>YNLDVRGARSFSPPRAGRHFGYRVLQVGNGVIVGAPGEGNSTGSLYQCQSGTGHCLPVTLRGSNYTSKYLGMTLATDPTDGSILACDPGLSRTCDQNTYLSGLCYLFRQNLQGPMLQGRPGFQECIKGNVDLVFLFDGSMSLQPDEFQKILDFMKDVMKKLSNTSYQFAAVQFSTSYKTEFDFSDYVKWKDPDALLKHVKHMLLLTNTFGAINYVATEVFREELGA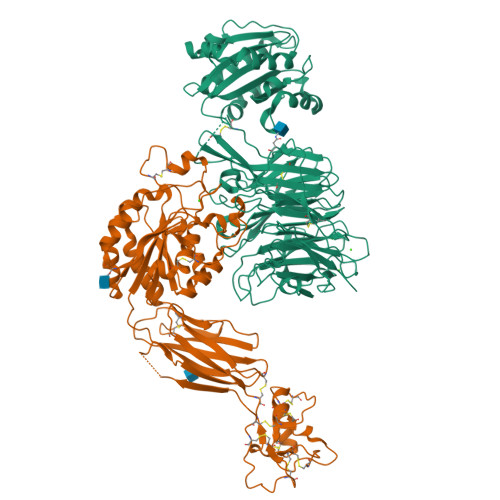RPDATKVLIIITDGEATDSGNIDAAKDIIRYIIGIGKHFQTKESQETLHKFASKPASEFVKILDTFEKLKDLFTELQKKIYVIEGTSKQDLTSFNMELSSSGISADLSRGHAVVGAVGAKDWAGGFLDLKADLQDDTFIGNEPLTPEVRAGYLGYTVTWLPSRQKTSLLASGAPRYQHMGRVLLFQEPQGGGHWSQVQTIHGTQIGSYFGGELCGVDVDQDGETELLLIGAPLFYGEQRGGRVFIYQRRQLGFEEVSELQGDPGYPLGRFGEAITALTDINGDGLVDVAVGAPLEEQGAVYIFNGRHGGLSPQPSQRIEGTQVLSGIQWFGRSIHGVKDLEGDGLADVAVGAESQMIVLSSRPVVDMVTLMSFSPAEIPVHEVECSYSTSNKMKEGVNITICFQIKSLIPQFQGRLVARLTYTLQLDGHRTRRRGLFPGGRHELRRNIAVTTSMSCTDFSFHFPVCVQDLISPIRVSLNFSLWEEEGTPRDQRAQGKDIPPILRPSLHSETWEIPFEKNPAALQTLFQGPLGAQGEKELQALEKENAQLEWELQALEKELAQHHHHHHA[3x];>QECTKFKVSSCRECIESGPGCTWCQKLNFTGPGDPDSIRCDTRPQLLMRGCAADDIMDPTSLAETQEDHNGGQKQLSPQKVTLYLRPGQAAAFNVTFRRAKGYPIDLYYLMDLSYSMLDDLRNVKKLGGDLLRALNEITESGRIGFGSFVDKTVLPFVNTHPDKLRNPCPNKEKECQPPFAFRHVLKLTNNSNQFQTEVGKQLISGNLDAPEGGLDAMMQVAACPEEIGWRKVTRLLVFATDDGFHFAGDGKLGAILTPNDGRCHLEDNLYKRSNEFDYPSVGQLAHKLAENNIQPIFAVTSRMVKTYEKLTEIIPKSAVGELSEDSSNVVQLIKNAYNKLSSRVFLDHNALPDTLKVTYDSFCSNGVTHRNQPRGDCDGVQINVPITFQVKVTATECIQEQSFVIRALGFTDIVTVQVLPQCECRCRDQSRDRSLCHGKGFLECGICRCDTGYIGKNCEPAALQTLFQGPLGAQGKKKLQALKKKNAQLKWKLQALKKKLAQHHHHHHA[3x]> MSGGTPEERLAQLEKEIQALYDAADEVVDEVEEKDGKMTVTRTLTIGDGTVTLVETLKIVD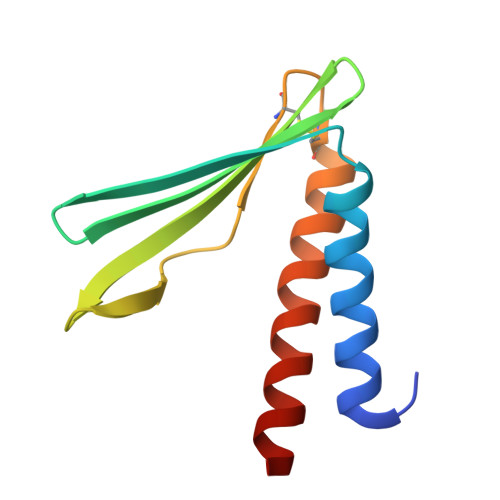GAPVKDGEIEVICNPECEELGKRLKALAKEYEKAQEEVEKAKA>[4x]MNKGVMRPGHVQLRVLDMSKALEHYVELLGLIEMDRDDQGRVYLKAWTEVDKFSLVLREADEPGMDFMGFKVVDEDALRQLERDLMAYGCAVEQLPAGELNSCG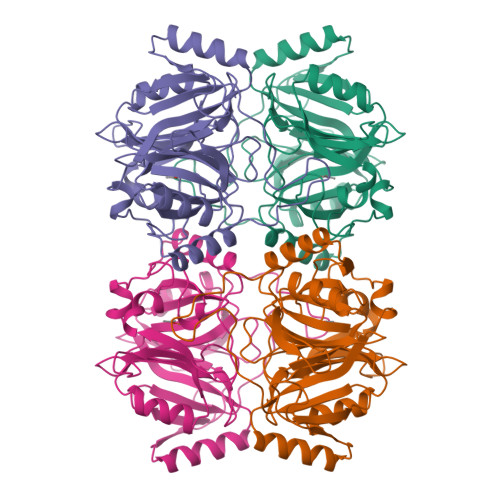RRVRFQAPSGHHFELYADKEYTGKWGLNDVNPEAWPRDLKGMAAVRFDHALMYGDELPATYDLFTKVLGFYLAEQVLDENGTRVAQFLSLSTKAHDVAFIHHPEKGRLHHVSFHLETWEDLLRAADLISMTDTSIDIGPTRHGLTHGKTIYFFDPSGNRNEVFCGGDYNYPDHKPVTWTTDQLGKAIFYHDRILNERFMTVLT> MWVYRLKGTLEALDPILPGLFDGGARGLWEREGEVWAFFPAPVDLPYEGVWEEVGDEDWLEAWRRDLKPALAPPFVVLAPWHTWEGAEIPLVIEPGMAFGTGHHETTRLALKALARHLRPGDKVLDLGTGSGVLAIAAEKLGGKALGVDIDPMVLPQAEANAKRNGVRPRFLEGSLEAALPFGPFDLLVANLYAELHAALAPRYREALVPGGRALLTGILKDRAPLVREAMAGAGFRPLEEAAEGEWVLLAYGR;> MKKVVAVVKLQLPAGKATPAPPVGPALGQHGANIMEFVKAFNAATANMGDAIVPVEITIYADRSFTFVTKTPPASYLIRKAAGL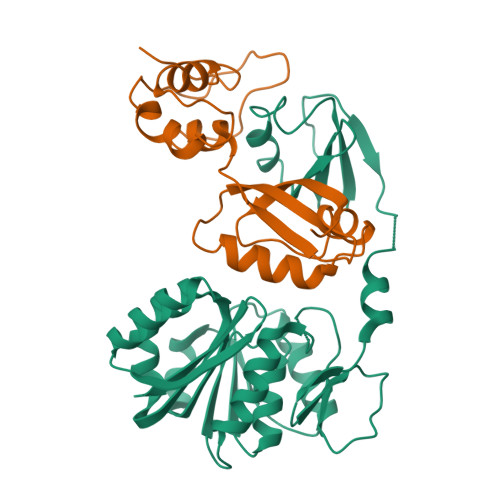EKGAHKPGREKVGRITWEQVLEIAKQKMPDLNTTDLEAAARMIAGSARSMGVEVVGAPEVKDA> SGSDGGVCPKILKKCRR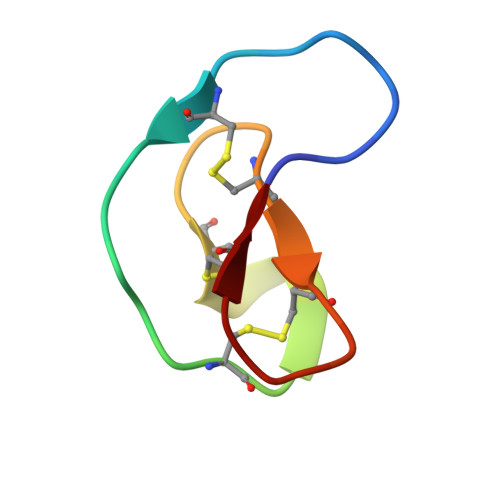DSDCPGACICRGNGYCG> QGLVDAMRGPT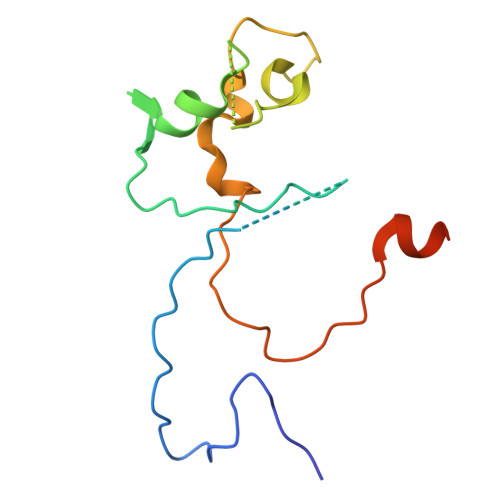AIANEPRAPLLYPTENKDIRRTRNYTMQPPTIPHKIDGYQLDKDFNRCMFCHARTRTEETQAIPVSITHYMDRDNNVLADVSPRRYFCTQCHVPQADTKPLIGNNFVDVDTILKRRPGAKGAAK>[2x]MAHHHHHHVDDDDKMVHHDGFQTVKATIDWEHPMFKLYEKAKRNGKWNPADIDFSQDQKDFASLTSEEKISALPLVAGFSAGEEALTLDILPMAHALARQGRLEDVLFLTTFMHDEAKHVEMFSRWQQAVGIGQMDLSVFHNDHY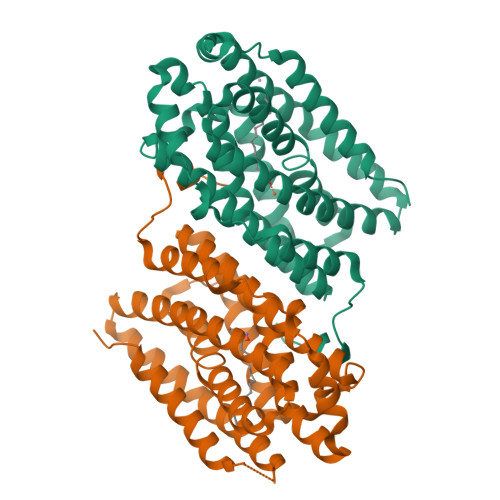KRIFYEALPEAMNRLYADDSPEAVIRAATVYNMIVEGTLAESGYYTFRQIYKKAGLFPGLLQGIDYLNMDEGRHIQFGIYTIQRIVNEDERYYELFIRYMDELWPHVIGYVDYLTELGKRQQQLARTYALEIDYDLLRHYVIKQFNLRKKQISRTKRVDVVEGLEKTAAES> MREYKLVVLGSGGVGKSALTVQFVQGIFVEKYDPTIEDSYRKQVEVDAQQCMLEILDTAGTEQFTAMRDLYMK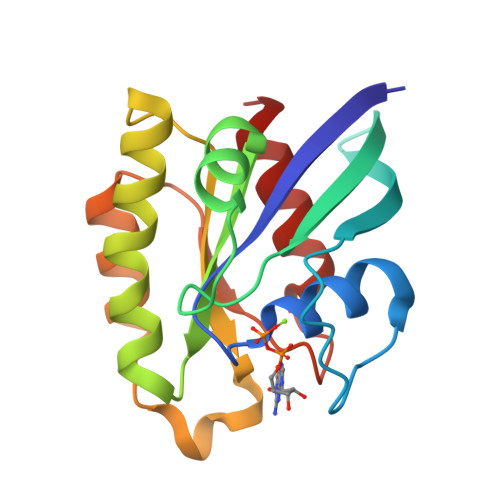NGQGFALVYSITAQSTFNDLQDLREQILRVKDTDDVPMILVGNKCDLEDERVVGKEQGQNLARQWSNCAFLESSAKSKINVNEIFYDLVRQINR6-(4-CHLOROPHENYL)IMIDAZO[2,1-B][1,3]THIAZOLE-5-CARBALDEHYDE O-(3,4-DICHLOROBENZYL)OXIME | C19 H12 Cl3 N3 O S | 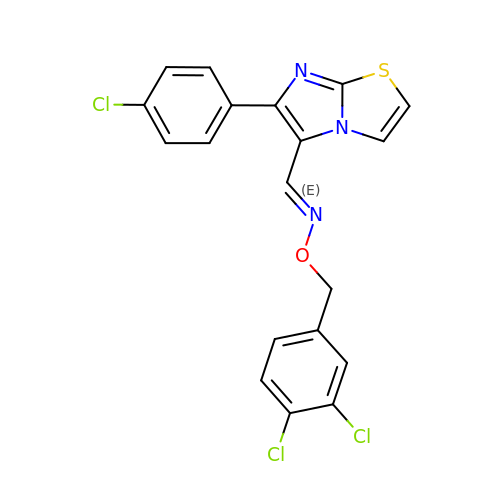ZQWBOKJVVYNKTL-AUEPDCJTSA-N In this program against the Mycobacterium tuberculosis (Mtb) cytochrome P450 CYP121 (the gene for which is essential for Mtb viability), overlapping fragments were found in both heme‐binding and non‐heme‐coordinating active‐site positions. Their elaboration via a fragment merging strategy proved highly successful for the heme‐binding fragments, but this was not recapitulated by compounds based on the non‐heme‐coordinating triazolylphenol fragment 1 (fragment 1­ KD=∼1.7 mm, merged fragment series 2–4­ KD=∼1–3 mm). Thorough investigation of the crystallographic active‐site complex, coupled with virtual screening, led to new structural scaffolds that were anticipated to alleviate the internal strain by subtly altering the ligands’ binding pose using a double hydrogen bond with a nearby Gln385 residue.

A clear possibility to enable such rotation was presented by the neighboring Gln385 residue on the opposite side of the narrow active‐site channel. We hypothesized that if an interaction with Gln385 could be strengthened (e.g., by using a double hydrogen bond)4 via subtle structural modification of 4, it could shift the restricted phenol sufficiently away from Val82 and Thr229 to return its rotational freedom, while still enabling 4 to maintain the other important interactions discussed above. The virtual screening results suggested that the 3‐aminopyrazole 5 would make the closest interaction with Gln385. Remarkably, 5 had a KD of 40 μm, 70‐fold greater than the original strained merged fragment 4, and a correspondingly high LE of 0.30 kcal mol−1 NHA−1 (NHA=non‐hydrogen atom). CYP121 crystals were individually soaked with aminopyrazole 5 and its analogues, leading to the successful determination of structures of 5 and 6 in complex with CYP121, both at 1.35 Å resolution. As predicted, compound 5 successfully positions to make a double hydrogen bond with the Gln385 side chain through its aminopyrazole. It also maintains all prominent interactions with the protein identified by 4, including one phenol hydrogen bonding to Asn85 and the other aromatic stacking between Phe168 and Trp182. The Gln385‐promoted interaction moves 5 sufficiently far from lying flat against Val82 and Thr229, such that there is a notable rotation in the originally constrained/restricted phenol adjacent to these residues (corresponding azole–phenol dihedral angles of 30° vs. 65° for 4 and 5, respectively). In silico QM calculations were performed for the conformational energetics of 5, which show that this rotation clearly alleviates the steric clash of the phenol ortho‐hydrogen atoms observed for 4. QM calculations (QM method: DFT(b3lyp), QM basis: 6‐31g**, gas phase) indicate no significant internal strain for the protein‐bound pose relative to the predicted ground‐state conformation in the gas phase (0.4 kcal mol−1).

> TATVLLEVPFSARGDRIPDAVAELRTREPIRKVRTITGAEAWLVSSYALCTQVLEDRRFSMKETAAAGAPRLNALTVPPEVVNNMGNIADAGLRKAVMKAITPKAPGLEQFLRDTANSLLDNLITEGAPADLRNDFADPLATALHCKVLGIPQEDGPKLFRSLSIAFMSSADPIPAAKINWDRDIEYMAGILENPNITTGLMGELSRLRKDPAYSHVSDELFATIGVTFFGAGVISTGSFLTTALISLIQRPQLRNLLHEKPELIPAGVEELLRINLSFADGLPRLATADIQVGDVLVRKGELVLVLLEGANFDPEHFPNPGSIELDRPNPTSHLAFGRGQHFCPGSALGRRHAQIGIEALLKKMPGVDLAVPIDQLVWRTRFQRRIPERLPVLW>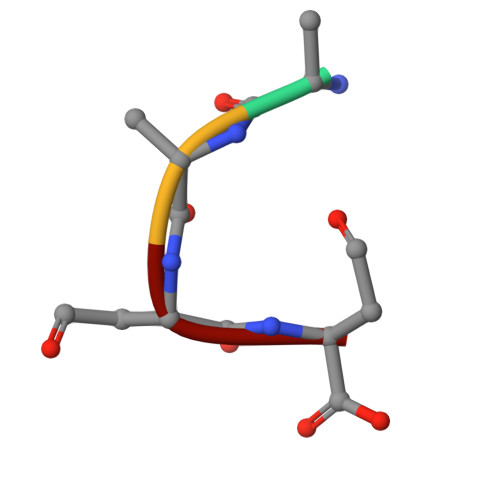 DDDD>[6x]MTETYPVVKGAEPFFFEGNDIGILVLHGFTGSPQSMRPLGEAYHEAGYTVCGPRLKGHGTHYEDMEKTTCQDWIDSVEAGYEWLKNRCGTIFVTGLSMGGTLTLYMAEHHPEICGIAPINAAINMP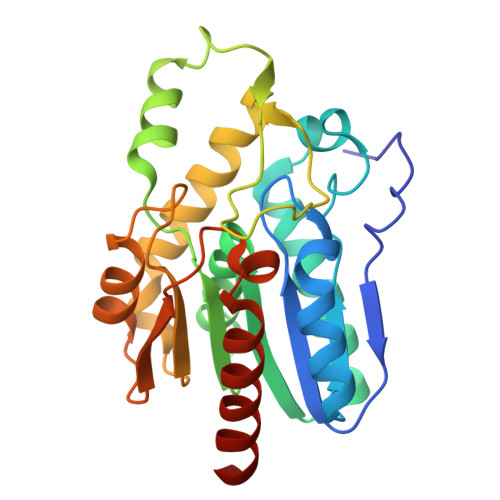ALAGALAGVGDLPRFLDAIGSDIKKPGVKELAYEKTPAASIRQIVQLMERVKTDLHKITCPAILFCSDEDHVVPPDNAPFIYDHIASADKKLVRLPDSYHVATLDNDRQKIIDTSLAFFKKHADRHHHHH heptachlor endo-epoxide 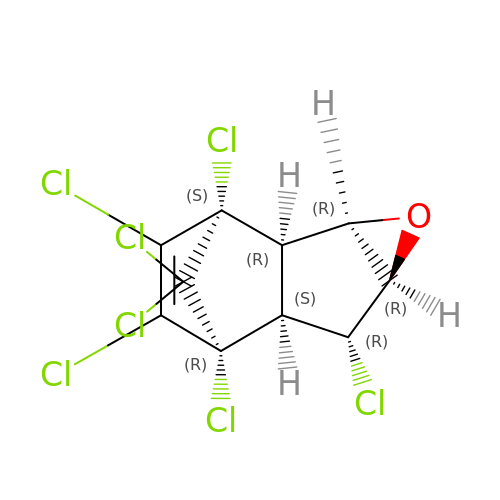| C10 H5 Cl7 O | ZXFXBSWRVIQKOD-WOBUKFROSA-N The Notch signalling pathway is conserved across all metazoan species and plays key roles in many aspects of cell biology including cell‐fate determination, stem cell maintenance, immune system activation and angiogenesis in humans (Guruharsha et al, 2012; Bray, 2016). Aberrant Notch signalling results in a number of inherited and acquired disorders, including various cancers, and it is therefore a key target for therapeutic intervention (Hansson et al, 2004; Groth & Fortini, 2012). Both the Notch receptors and the ligands are single‐pass type I transmembrane proteins, and direct protein–protein contact between adjacent cells initiates an intracellular signalling pathway. All of the Notch ligands have a modular extracellular architecture consisting of an N‐terminal C2 domain (formerly known as the MNNL domain), a Delta/Serrate/Lag‐2 (DSL) domain, and either 16 (Jagged1/Jagged2), 8 (Delta‐like1/Delta‐like4) or 7 (Delta‐like3) EGF repeats. Binding of a Notch ligand to EGF11‐12 of a Notch receptor results in a series of proteolytic cleavages, with the final intra‐membrane cleavage by gamma secretase, causing the release of the intracellular domain of Notch (NICD) from the plasma membrane.

Here, we present the first structures of Jagged2 (N‐EGF2 and N‐EGF3), which has only 58% sequence identity with human Jagged1 (N‐EGF3), together with the longest known structure of a Delta‐like4 ligand (human Delta‐like4 N‐EGF3). Two crystal forms of Jagged2 (N‐EGF2) (green) and one crystal form of Jagged2 (N‐EGF3) (dark green) were solved, including a total of seven crystallographically independent copies of N‐EGF2, and 1 copy of N‐EGF3 (N.b. not all of EGF3 is visible in the electron density). All of these copies have been superposed on each other by alignment of the DSL domain, showing some flexibility in the hinge region between the C2 and DSL domains, and further flexibility in the hinge regions between the EGF domains. The Jagged1 and Jagged2 C2 domains bind calcium ions (shown in red), whereas Delta‐like4 and Delta‐like1 do not; the aspartates involved in calcium binding are not conserved in Delta‐like4 and Delta‐like1. The C2 loops are ordered upon calcium binding in both Jagged1 (Chillakuri et al, 2013) and Jagged2 and contain the amino acid ligands for calcium binding although the number of calcium ions bound differs. Interestingly, the three calcium ions bound in the Jagged2 C2 domain are at equivalent positions to three of the five calcium ions bound in the Perforin C2 domain (Yagi et al, 2015). The α(1,6)‐linked fucose on the Asn‐153 N‐glycosylation site in Jagged2 packs against Trp‐151 side chain (shown).

> MGYFELQLSALRNVNGELLSGACCDGDGRTTRAGGCGHDECDTYVRVCLKEYQAKVTPTGPCSYGHGATPVLGGNSFYLPPAGAAGDRARARARAGGDQDPGLVVIPFQFAWPRSFTLIVEAWDWDNDTTPNEELLIERVSHAGMINPEDRWKSLHFSGHVAHLELQIRVRCDENYYSATCNKFCRPRNDFFGHYTCDQYGNKACMDGWMGKECKEAVCKQGCNLLHGGCTVPGECRCSYGWQGRFCDECVPYPGCVHGSCVEPWQCNCETNWGGLLCDKDLNGSHHHHHHHH> QDADKLPHTKVTLVAPPQVHPHEQATKSGPKVVEFTMTIEEKKMVIDDKGTTLQAMTFNGSMPGPTLVVHEGDYVQLTLVNPATNAMPHNVDFHGATGALGGAKLTNVNPGEQATLRFKADRSGTFVYHCAPEGMVPWHVVSGASGTLMVLPRDGLKDPQGKPLHYDRAYTIGEFDLYIPKGPDGKYKDYAT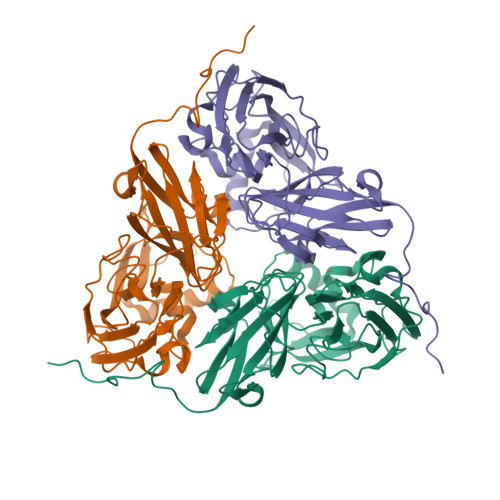LAESYGDTVQVMRTLTPSHIVFNGKVGALTGANALTAKVGETVLLIHSQANRDTRPHLIGGHGDWVWETGKFANPPQRDLETWFIRGGSAGAALYTFKQPGVYAYLNHNLIEAFELGAAGHIKVEGKWNDDLMKQIKAPAPIPR> AQSVPYGVSQIKAPALHSQGYTGSNVKVAVIDSGIDSSHPDLKVAGGASFVPSETNPFQDNNSHGTHVAGTVAALDNSIGVLGVAPSASLYAVKVLGADGSGQYSWIINGIEW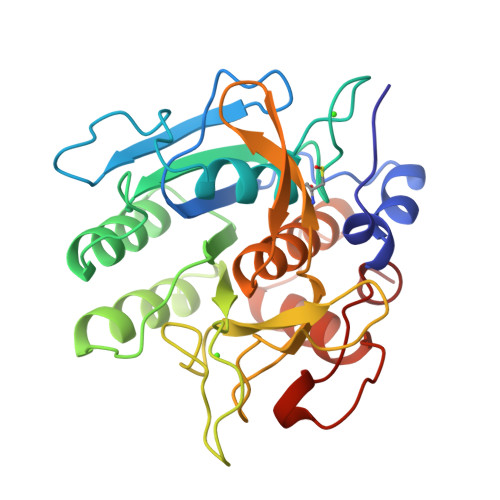AIANNMDVINMSLGGPSGSAALKAAVDKAVASGVVVVAAAGNEGTSGSSSTVGYPAKYPSVIAVGAVDSSNQRASFSSVGPELDVMAPGVSICSTLPGNKYGAYSGTSMASPHVAGAAALILSKHPNWTNTQVRSSLENTTTYLGDSFYYGKGLINVQAAAQ> SQIPASEQETLVRPKPLLLKLLKSVGAQKDTYTMKEVLFYLGQYIMTKRL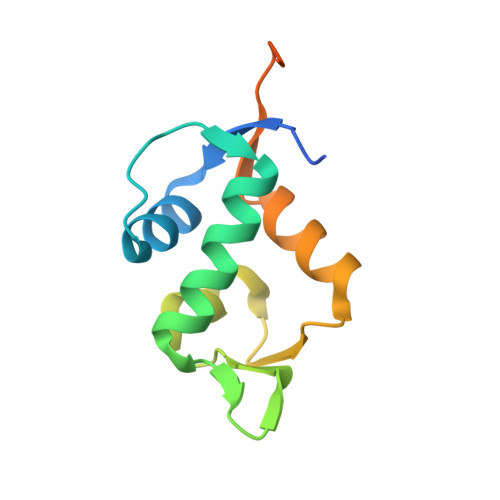YDEKQQHIVYCSNDLLGDLFGVPSFSVKEHRKIYTMIYRNLVVVNQQESSDSGTSVSENHHHHHH>[2x]ATKKAVAVLKGNSNVEGVVTLSQDDDGPTTVNVRITGLAPGLHGFHLHEY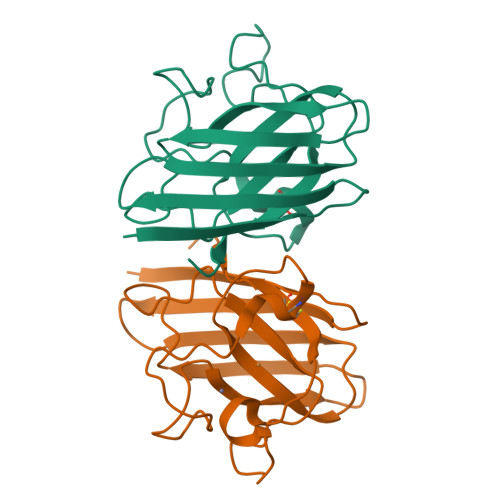GDTTNGCMSTGAHFNPNKLTHGAPGDEIRHAGDLGNIVANADGVAEVTLVDNQIPLTGPNSVVGRALVVHELEDDLGKGGHELSLTTGNAGGRLACGVVGLTPI> SSESTTFIVDVSPSMMKNNNVSKSMAYLEYTLLNKSKKSRKTDWISCYLANCPVSENSQEIPNVFQIQSFLAPVTTTATIGFIKR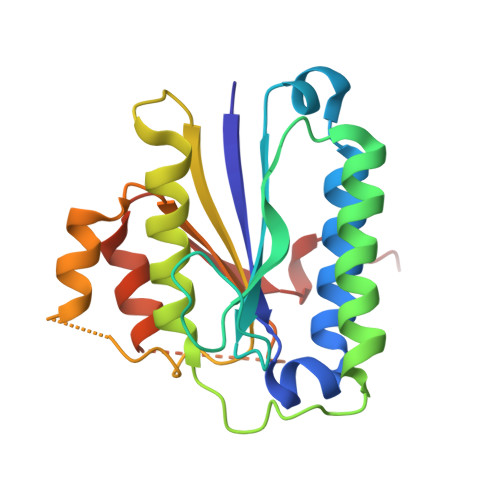LKQYCDQHSHDSSNEGLQSMIQCLLVVSLDIKQQFQARKILKQIVVFTDNLDDLDITDEEIDLLTEELSTRIILIDCGKDTQEERKKSNWLKLVEAIPNSRIYNMNELLVEITS> SASGVDDRDLLLAPKWISFLSLSSFLKQKLLSLLRQIRELRLTTTVYPPQDKLMWWSHCCDPEDIKVVILGQDPYHKGQATGLAFSVDPQCQVPPSLRSIFRELEASVPNFSTPSHGCLDSWARQGVLLLNTVLTVEKGRAGSHEGLGWDWFTSFIISSISSKLEHCVFLLWGRKAIDRT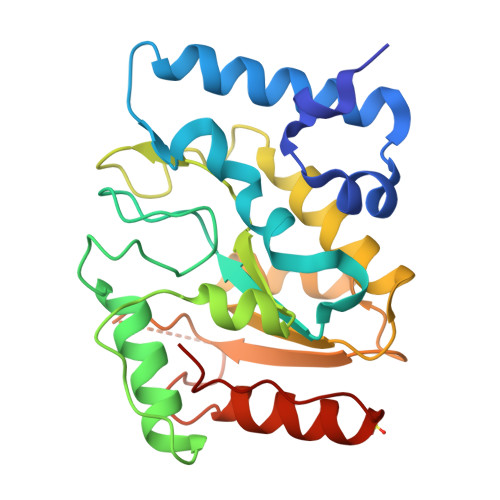PLINAQKHLVLTAQHPSPLASLGGRHSRWPRFQGCNHFNLANDYLTRHRRETVDWGLLEQ> SANEDMPVERILEAELAVEPKTETYVEANMGLNPSSPNDPVTNICQAADKQLFTLVEWAKRIPHFSELPLDDQVILLRAGWNELLIASFSHRSIAVKDGI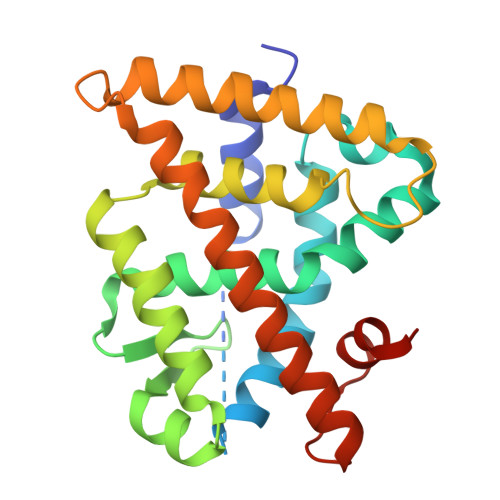LLATGLHVHRNSAHSAGVGAIFDRVLTELVSKMRDMQMDKTELGCLRAIVLFNPDSKGLSNPAEVEALREKVYASLEAYCKHKYPEQPGRFAKLLLRLPALRSIGLKCLEHLFFFKLIGDTPIDTFLMEMLEAPHQMT>[4x]GSMKFEFENRTLVLTGANGGIGRAIAELFHASGANLVLTDLDREGLDAFAASLGSPERIATIKADASSADDAEKTVALAMERFGGIDFLVPSAGIYQAKPFAEMSDADWHRTISINL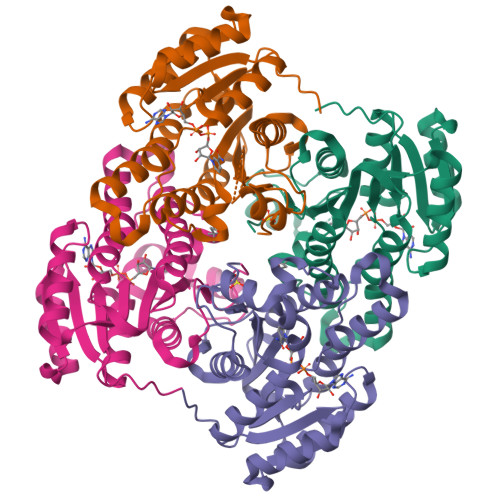DGVFYLCKRALPALKEDSSIVTLASLAAYRGAYVNAHYGATKGAMVSMTRALSRELAPKTRVNGVSPGIIETPMTSELLKTRMDETMTQTPLKRLGKPSEIASVIAFLCSPAASFVTGETIQVNGGIYMA> MKLYSLSVLYKGEAKVVLLKAAYDVSSFSFFQRSSVQEFMTFTSQLIVERSSKGTRASVKEQDYLCHVYVRND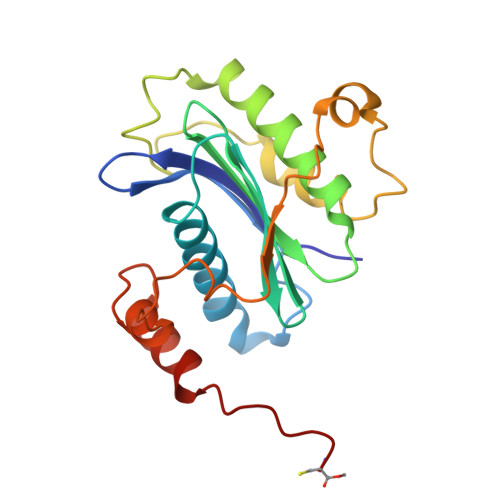SLAGVVIADNEYPSRVAFTLLEKVLDEFSKQVDRIDWPVGSPATIHYPALDGHLSRYQNPREADPMTKVQAELDETKIILHNTMESLLERGEKLDDLVSKSEVLGTQSKAFYKTARKQNSCC>[8x]MSKKLTTAAGCPVAHNQNVQTAGKRGPQLLQDVWFLEKLAHFDREVIPERRMHAKGSGAYGTFTVTHDITKYTKAKIFSDIGKKTDMFARFSTVAGERGAADAERDIRGFSLKFYTEEGNWDLAGNNTPVFFLRDPLKFP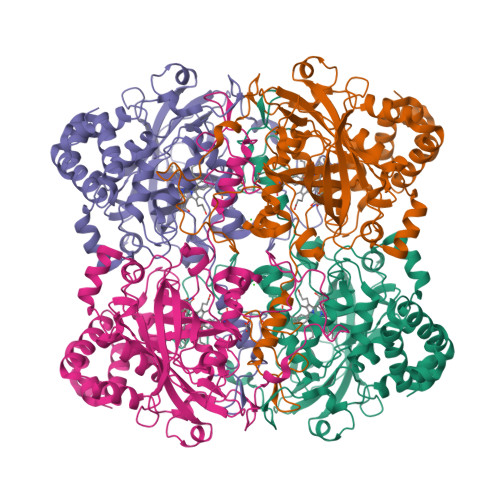DLNHAVKRDPRTNMRSAKNNWDFWTSLPEALHQVTIVMSDRGIPATYRHMHGFGSHTFSFINSDNERYWVKFHFVSQQGIKNLSDAEAGELVGNDRESHQRDLLDSIDNQDFPKWTLKVQIMPEADAATVPYNPFDLTKVWPHKDYPLIEVGEFELNRNPQNYFAEVEQAAFNPANVVPGISFSPDKMLQGRLFAYGDAQRYRLGVNHQHIPVNAPRCPVHSYHRDGAMRVDGNFGSTLGYEPNDQGQWAEQPDFSEPPLNLDGAAAHWDHREDEDYFSQPGDLFGLMTAEKQAILFDNTARNLNGVPKEIQLRHVTHCYKADPAYGEGIGKLLGFDISEYNS>[10x]MKADNPFDLLLPAAMAKVAEEAGVYKATKHPLKTFYLAITAGVFISIAFVFYITATTGTGAMPYGMAKLIGGICFSLGLILCVICGADLFTSTVLIVVAKASGRITWGQLAKNWLNVYFGNLIGALLFVLLMWLSGEYMTANGQWGL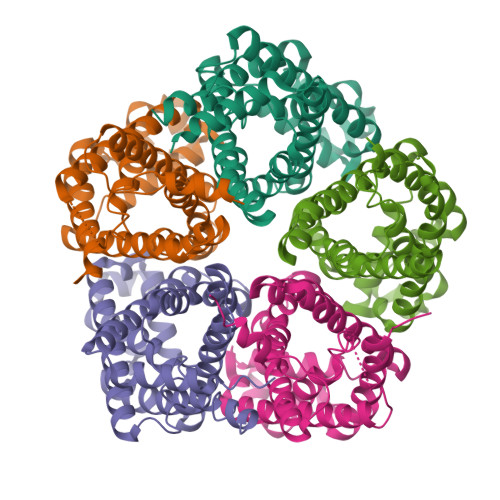NVLQTADHKMHHTFIEAVCLGILANLMVCLAVWMSYSGRSLMDKAFIMVLPVAMFVASGFEHSIANMFMIPMGIVIRDFATPEFWTAVGSSPESFSHLTVMSFITDNLIPVTIGNIIGGGLLVGLTYWVIYLRGNEHHLEHHHHHH> MGSDKIHHHHHHENLYFQGMEIKEYENNPYHLAQLVDLINYCQNIEAKLDIKMAEQDDIFQIENYYQNRKGQFWIALENEKVVGSIALLRIDDKTAVLKKFFTYPKYRGNPVRLGRKLFERFMLFARASKFTRIVLDTPEKEKRSHFFYENQGFKQIT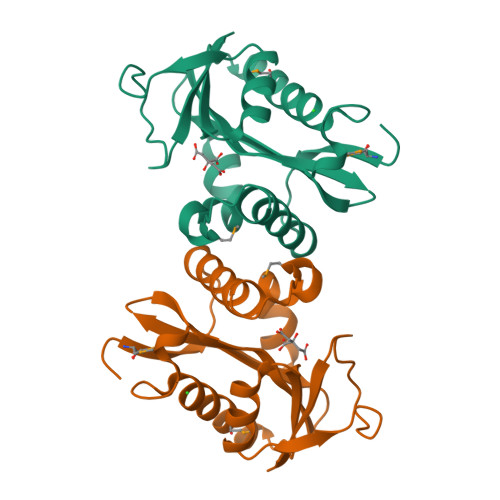RDELDVDYIFPDRDSRIYVKLLD> LPTSNPAQELEARQLGRTTRDDLINGNSASCADVIFIYARGSTETGNLGTLGPSIASNLESAFGKDGVWIQGVGGAYRATLGDN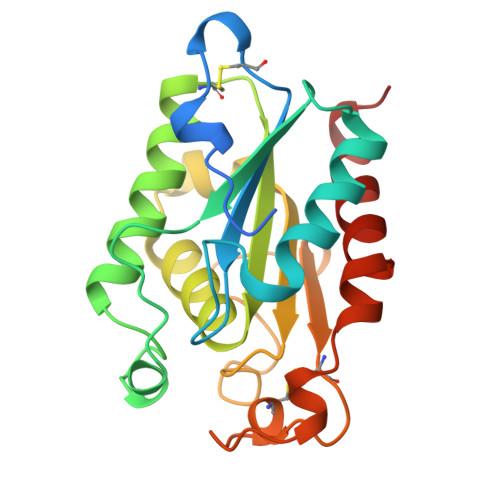ALPRGTSSAAIREMLGLFQQANTKCPDATLIAGGYSQGAALAAASIEDLDSAIRDKIAGTVLFGYTKNLQNRGRIPNYPADRTKVFCNTGDLVCTGSLIVAAPHLAYGPDARGPCPEFLIEKVRAVRGSA> MGSSHHHHHHSSGLVPRGSLKGNIRVFCRVRPVLPGEPTPPPGLLLFPSGPGGPSDPPTRLSLSRSDERRGTLSGAPAPPPRHDFSFDRVFPPGSGQDEVFEEIAMLVQSALDGYPVCIFAYGQTGSGKTFTMEGGPGGDPQLEGLIPRALRHLFSVAQELSGQGWTYSFVASYVEIYNETVRDLLATGTRKGQGGECEIRRAGPGSEELTVTNARYVPVSCEKEVDALLHLARQNRAVARTAQNERSSRSHSVFQLQISGEHSSRGLQCGAPLSLVDLAGSERLDPGLALGPGERERLRETQAINSSLSTLGLVIMALSNKESHVPYRNSKLTYLLQNSLGGSAKMLMFVNISPLEENVSESLNSLRFASKVNQC

Kinesin motor proteins hydrolyze ATP to produce force and do work in cells. Despite their diverse functions, the kinesin proteins contain a common motor domain with highly conserved or invariant sequence motifs that mediate basic motor properties, such as microtubule binding and ATP hydrolysis. For example, kinesin-14 motors move on microtubules towards the minus end instead of the plus end. Here we report a new crystal structure of human kinesin-14 KIFC1, together with new crystal structures of Drosophila Ncd, a KIFC1 orthologue, and human KIFC3, a divergent KIFC1 paralogue, and an analysis of the structural features of the proposed KIFC1 AZ82 inhibitor-binding site.

The new KIFC1 (2.25 Å) and KIFC3 (1.85 Å) structures were determined by the Structural Genomics Consortium. Both proteins were crystallized bound to Mg-ADP and are reported here for the first time. Despite its importance as a potential drug target, this is the first KIFC1 structure to be determined and the only one available to date. Comparison of KIFC1 to Ncd shows that the two motors are structurally very similar to one another with differences in loops, which are longer in KIFC1 than Ncd H1 or H2, as predicted above. In order to evaluate the ability of the KIFC1 L5/α2/α3 pocket to bind small molecules, we superposed our KIFC1-ADP crystal structure with kinesin-5-ADP-ispinesib. Viewed from the nucleotide-binding side of the motor, the ribbon diagram of the superposed structures shows the KIFC1 helix α3 tilted inward towards helix α2, reducing the size of the pocket in KIFC1 (Fig. 2A Center; KIFC1 L5/α2/α3, pale blue). A critical residue of KIFC1 relevant to formation of the L5/α2/α3 pocket is R521 of helix α3, which is positioned under loop L5 (Center, hot pink). Interaction of the side chain of R521 with other residues stabilizes L5 and maintains the closed conformation of the potential binding pocket, disfavoring binding by small molecule at the site. The KIFC1 conformation with the highest predicted AZ82 free energy change shows movement of residues, including Y409, L599 and F656, to form the binding site. The movement of F656 allows the hydrophobic AZ82 F3 group to become buried deep in the KIFC1 α4/α6 pocket, which is likely to stabilize AZ82 binding.The Staphylococcus aureus pathogenicity islands (SaPIs) are the prototypical members of the phage-inducible chromosomal island (PICI) family of mobile genetic elements. Stl is a DNA-binding protein that binds to the intergenic promoter region between stl and str (the SaPI transcription rightward regulator), preventing transcription of the str and downstream genes, thus maintaining integration of the island in the host chromosome. The remarkable ability of the SaPIbov1 Stl to target unrelated but functionally similar antirepressor proteins relies on the modularity of this repressor. In this way, SaPIbov1 Stl presents three domains: one corresponds to an HTH N-terminal domain required to recognize and bind the divergent stl-str region present in the SaPI genome; a second (middle) domain responsible for interacting with the trimeric Duts, while the C-terminal part of the protein recognizes the dimeric Duts.

Therefore, we determined to solve the structure of BovI-Stl by eliminating this region and dividing the protein into two functional and complementary portions corresponding to the N-terminal (BovI-StlN-ter; residues 1–156) and to the C-terminal part of the protein (BovI-StlC-ter; residues 175–267). The crystal structure of BovI-StlN-ter was solved to 1.8 Å resolution and showed a single copy of the protein in the asymmetric unit that presents an α-helical folding, as was anticipated by in silico modelling, composed of 10 α-helices. The initial four α-helices (α1–α4) correspond to the DNA-binding domain, presenting the archetypical helix-turn-helix (HTH) motif observed in multiple repressors, as well other DNA-binding proteins. Helix α5 connects the HTH domain with the remaining five helices that form a more compact helical bundle. We named this portion of the protein the middle domain due to its localization in the Stl sequence. The structure shows that the N-terminal and middle domains are closely connected by helix α5, while an unstructured region of about 20–30 residues connects the middle and C-terminal domains. In the model, BovI-Stl recognizes the DNA by inserting helix α3 of the HTH motif into the major groove of DNA. Our model further proposes that additional residues such as Q29, S44, N48 and R22 could mediate the nonspecific read-out of the nucleotide sequence by interacting with the DNA backbone. The first three residues coordinate a sulfate ion in the BovI-StlN-ter structure that could mimic a DNA phosphate, since superimposition with the C.Esp1396I-DNA complex places this sulfate at the position of a DNA backbone phosphate.

> GMEGAGQMAELPTHYGTIIKTLRKYMKLTQSKLSERTGFSQNTISNHENGNRNIGVNEIEIYGKGLGIPSYILHRISDEFKEKGYSPTLNDFGKFDKMYSYVNKAYYNDGDIYYSSYDLYDETIKLLELLKESKINVNDIDYDYVLKLYKQILSTDT Nuclear pore complex (NPC) constitutes the only regular route of cargo transport between the cytoplasm and the nucleus. The vertebrate NPC, with a combined molecular mass of over 100 MDa,11–13 consists of three central ring scaffolds that collectively define the central pore: cytoplasmic ring (CR), inner ring (IR), and nuclear ring (NR)4,9,14,15. CR and NR share a similar overall organization and are characterized by a conserved set of nucleoporins. Here we present single-particle cryo-EM structure of the nuclear ring (NR) subunit from Xenopus laevis NPC at an average resolution of 5.6 Å.

The structurally resolved NR subunit contains 22 molecules of 12 distinct nucleoporins, one molecule each for Nup205/Nup93 and two molecules each for the other 10 nucleoporins. Each Y complex comprises a short arm (Nup85, Nup43, and Seh1), a long arm (Nup160, Nup37, and ELYS), and a stem (Sec13, Nup96, Nup107, and Nup133). Compared to the CR, each Y complex in the NR contains an additional nucleoporin ELYS, which closely associates with Nup160 and Nup37 in the long arm. In our structure, the N-terminal β-propeller of inner ELYS stacks against the N-terminal β-propeller of inner Nup160; the α-helical domain of inner ELYS aligns with the α-helical domain of inner Nup160, orienting the AT-hook domain into the nucleoplasm. Through close interactions with Nup160 and Nup37, ELYS becomes an integral component of the long arm of the Y complex in the NR subunit. Notably, inner ELYS from one NR subunit also bridges interaction with an adjacent NR subunit. Unlike the CR subunit, the NR subunit contains only one molecule of Nup205, which corresponds to outer Nup205 in the CR subunit. Similar to that in the CR subunit, Nup205 in the NR subunit interacts with the short arm and the vertex of outer Y complex; it also associates with both arms of inner Y complex. Unlike that in the CR subunit, the NR subunit only contains one molecule of Nup93, which interacts with both stems of the inner and outer Y complexes. Nup93 connects the stems of inner and outer Y complexes within the same NR subunit, and places its N-terminal extended helix into the axial groove of Nup205 from the neighboring subunit.

> MAAQLALNSEASLWGPYREIWQTVLSALIKRQPEAVHSLDIVLKKYKPDFISLFKNPPKSAQQHERVQKASTEGIPIKGTQRTRILEEQLIKEAFILSDLYNIGEIAAVELLLIGEQQQPTFHGLTRGLVAILLYWDGKSCMAESLLHLIQARKGKTFTLDHSPEVVSMVTRFTDDLMEQGLTNKILTLISQIDVNNEFDKLKKERGLGNKKHRKEVSDLIKECQQSLAHSLYSWSCQTPLNREDTLLLIGYLEKVTVEGDGSLDKVNLTLLMSLLYCLDVGFLEQGTDDREELMKQASMFMDRQYIAAIHNRLQNTQPWKSPGMQATVRLAWALALRGISQFSEVLEFSEADEPMAEIAIGGNVFLFLTEAVVGSESFCTDEFFIRRIHKLVTDFPTLMPMKVKQLRNRAEEDARLIQMSMQMGNEPPASLRRDLEHLLLLIGELYRKDPFHLELALEYWCPTEPLQSTSLMGSFLGVAHQRPPQRQVLLSKFVRQMSDLLPATLYLPYLKMLRGLASGPQCAHYCFSLLKANGGSSAENLQAAGGSPVSWDHFFHSLMLYHEHLRRDLPNTDNIHQRHPPLRGITQRELDGLIACLQLTCTIIDWSESARLALCEHAQWMPVVVILGLLQCSIPPLLKAELLKTLAAFGKSPEIAASLWQSLEYTQILQTVRATGLRQGVGIEVELNEIESRCEEYPLTRAFCQLISTLVESSFPTNLGAGLRAPGFEPYLQFLRDTVFLRYRTRAYRRAAEKWEVAEAVLDVFYKLLKDYEPQPEDFVDQYVELQGEERVAFKPPGFSLMHHLLNESPMLELCLSLMEEGVTQLDTYAPFPGKKHLEKAVAYCFMLLNLTLQKENRFMDLLRESHLSMIVTPLEQLLQGINPRSKKADNVVNIARYLCHGNSNAELAFESAKILCSISCNSKIQEKIVGDFTQDQNVSQKLMVGFVSCLDSEEAEELLDSEKEAEDQVKQTNIRYMTKIHILNLLITSLEMKAPNLAMFLLGYELKKPVSTTNLQDSGVLGCPRTCLHSILDILRKGTDVRAGPVAVWDTPHLAELCYQVIYQLCACADTSGPTMRYLRTSQDFLFSQLQHLPFSVEESEISAMNQMSWLMKTATIELRITSLNRQRSHTQRLLHLLLDDMPTRPYSADGEGGMEDESRSLSGFLHFDTTSKVRRKILRILDSIQFSNEIPEPLQLDFFDRSQIEQVIANCEHKNRRGQTVCNVKLLHRVLVAEVNALQGMAAIGQRPLLMEEINTILQYVVERNKLLQCLHAKRHALESWRQLVEIILTACPQDLIPTEHRQLIIRDLLQDLHVKILDDDAAQELMPIVAGAVFTLTAHLSQSVRTELKQPMTASGLGQSQYVQMLDGSFAAPPGTENISAGFASIGDSSLHMILRNLLEFILKTGGGFQRVRAHLYGSLLYYLQIAQRPDEPDTLESAHKSMWERLTAPEDVFSKLQRDNLSIFESYGTALMEVVCRDACDGHDIGRMLALALLDRIVSVDRQQQWLLYLSNSGYLKVLVDSLAEDDVVLRNLLTPQPPLLKALYIYESKMAFLTRVAKSSQGAIELLRSGVIVRLAQCQVYDMRPETDPHGVFGMRETPVFIPAPVERYRQILLPALQICQLILTSSTAQHLQAAGQVLQFLVAHSDTIQAILRSQEGSLGSLQELALLTGIISKAALPGVLNELDIGLNDGSMMELQGHIGRFQRQCLALLNRFGGSDRLRQLSLQDDSSRLDGVSKKDDMELAMQQICSNVMEYCQALMIQNSPSFQQTVCLFTPSLKESASRDGTRQDSQVSILPSWRLPSLGVVIHLLKQSANNFFTYYDIHRQSVGKLQNVEQLPPDEIKELCQSEMPVGADKISTTQKYGLARRRLVKLINSRAKLLSLCSYIIETCLYILWRHLEYYLLHCTTSDSQDPVFSNMTFGNRRFQDTFNTDPNMDPRNLRQNKVSQQDVDTLLREGANSFGESLQKRLLDIESLYCKVRSRHSFIQALVRRIRGLLRVSRV;>MEELDVDPAETPIPGLGQQNRHIGFSWGPGDLLLYETLYQKQGNSETAARCPFMYLVRSDEDIYSPVLRKLFNESHSIFVGLQKSAEEASGKSRKAQLVQVSRNYRSVLRACMEEMHTLSESTRETAQKYISQISILSAMELSWNLCEILFIESAPAGPLLILLLEWVRLHVCEVDNIVQDVLRSEKPTEHEKFWDGVTGYVLQGRMNEARQLLAKEASTSASARSMCRVLDDLLKKMPMLHTGGTQTLTEFELKWQHWREECERHLQNGTFSSNVHMEAVCRVLLGDEEVLLEKRDLMTTWYHFLVSRLLFKHPTVKPTELHFYAQSSLDMFLAGDSCPEPLDNILLAAFEFDIHQVIKEFSIVSSNWWFVAHLTDLLDHCQLFQAHNLYFGANMREFLLLDYASGLFSHHSLWQLGVDYFDYCPNLGREYLKLHMERIPLSTEKKALKALRICEQRQMTEQVRSICKTMAMQSLCNRRLGSALSWSIRAKDAAFATLISDRFLKEYCERGNFTDLDLIDNLGSAMLLSDRLTFLGKYREFHRMYSQEQFSEAASLLLSLMTARIAPCSFWLTLLLDALPLLEQKQVIFSAEQTYELMRCLEDRMAAKLESTSPDEIQKQDSSIDNTKVEMLRLALARNLARAIVTEGALQE[2x];>MADKFAAKFVSHKISRTRWRPVSASSLQQPDVFATGSWDNEENKVCVWATSDFGATSLDEEYQGDPKQLCDIKHPGDVMDMQFLDKERIVTGSSTGTVTIFRHHENNQTLSVNQRWEQAHYHVGSNMRAPCTAIVCSSPEIVSVGEDGRINCFRAESRDVLRTIDDADSSTMHGVTFLRTTEILTVNSVGQLKLWDLRKQGNDPTQIFSVTGERVPLHCVDRHPNQQHVVATGGQDGMLCIWDVRHGKMPMSLLNAHEAEMWEVHFHPSNPDHLFTCSEDGSLWHWDASADSEKPTFLLGGRSTFNISRSSIAPPNANQSLACAWLSTDPTKGQLEITNLLPSSTLSVNSLDVLGQNLVCGTDAEAIYVTRRLFS[2x];>[2x]MFVARSIAADHKDLIHDVSFDFHGRRMATCSSDQSVKVWDKSENVNWHCTASWKTHSGSVWRVTWAHPEFGQVLASCSFDRTAAVWEEIVGESNDKLRGQSHWVKRTTLVDSRTSVTDVKFAPKHMGLMLATCSADGVVRIYEAPDVMNLSQWSLQHEISCKLSCSCISWNPSSSRAHSPMIAVGSDDSSPNIMGKVQIYEYNENTRKYAKAETLMSVSDPVHDIAFAPNLGRSFHILAVATKDVRIFTMKPLRKELSSSGGVTKFENHTVAQFDNHNSQVWRVSWNITGTVLASSGDDGTVRLWKANYMDNWKCIGVLKGDGNPVGNSFQGIFGSSIGSASHGLQNSVNGTSTSGRKHS;>MAAAERHMTPFQAIDWAGSITLPMVQRVGGFTRAIMAASVNLERSYMELIGAERETSRRNFRDLSLRPDVNLVIGGPKYADCAGGYCYSESSSLLSATRNRFLHWTSYADTLELVEISLDINLVNNAVRLRILNCSILPGGVHICETPNNIVVLILTNQTVHRLILPHPSRMYRSEIISDSHIQSIFTDIGKTNFHDPSNTYVIPAIPGRAPNTTASTAWLSSDGEALFALPSISGGILVIKMPPHDMEGLVTIAELKQSSVMQRLLTGWMPSSIRGDQGPAHLPVSLAVHTLDHDSYLFALCQDHKLRMWSYKDQMCLMVADMLEYVPVSKDIRQTAGTGHKLRLAFSETLGILYLGVYLHTPKQGQFCVFQLMCAESNRYSLDHISSIFTNQETLIDFTFTLTSMDIWALWLDDDNQTVVKHINFEENQAGQWNPVFVNPLPEDDLAISDEQEPQEAYLECLFAPGRFTIAAVQKAIQILRKGSGRVLDLSWEELRKDVTLTVENEIQNAVIDYDVSQEEFRQINIENWCKFYTCCLQYQETLSRPLALLVHPDTNMVCLLRKGFLSFLAPCSLVEHLYLVPAEHLLTVDESVISDDIDAASDIVNLIQCLRMIADYISEDMAYLMESACCHLQSPERVAEQILEDLIANDIDNIMENIQNKLQDTRNPIRAIGFLLQNMDYETNADMEQPQPNTRLNLSTLYGSITASSVVCQAICKISATRFLICRDLLILQHLLLRLGDMALIGAGQLLHSQQELIPRAAQLLLSYYMIRWGSQCLACAVPVDILESNLQHLSVLELSDSQVEKRRYTSGIQTIVELFFEDVARKHFPHVFIQSGASQLQEPLNWSDLIKRITNYLLQLLWPSNPNFQFAECLMRNCQYTQLQEYVRLLLPWCQVNVGSCHFMLAQCYLVAGEGHKALDCFSQAASEVEREDFLEKLIRVEEGESVSPRLQYYNRVLRLLEDVGLPELVIQLATIAIGEASDDWRSQAALRTRIFKHHLDMGHNNQAYDALTQIPDPSRQLDCLRQLVVVLCERSQLQDLVEFPYVNLHNEVVGIIESRARAVDLMTHNYYELLYAFHIYRHNYRKAGSVMFEYGMRLGREVRTLRGLQKQVNSYLACLNCLRLIRPEYAWIVQPVSGAVYERPGASPKRNYDGESSAVPSSSQIEILELRDLEKEYVLAQTRLTLAKHNPSTAAIAGSSAAEEMVALLVQAGLFDTAISLCQTFKLALTSVFEGLACKCIRLQQGGEAAQAEAWEWLAANQLATVITTKESSATDEAWRLMISYLDKYEAKNTLYHHCIINKLLSHGVPLPNWLINRYKAMDAAELLRLYLKYDLLEEAAELVLEYVDALLGKGHQYFGIQAPLSATSQLVWFPYSAIDHLRQALGENESNQHNQAILSKLQRKMDEYFQKLKKATDDYKKLVQKPLRA[2x];>[2x]MKQDSASNATYTVDCEDYVHVVEFNPFDSGEAGSLLAYGGISYVVIASCRFQEEDSTVEGIEFKTLKTFHHGERVVAIAWSPETRCDALLPLLRFATAAGDKKIRIFTSDFQDKNEYKVIEGHSGYINDLVFCSPEGTDIASVGDDHTCRIWDLDGKQIAMFILRSPGMSVAWHPEGAFKLMVAEKTGTIRFYDLTTHQAILSLESVQVPLMSADWCVRNTLRIGAVAGNDWIIWEMPRSSYPQDNKPAHADRARMFRWSKCNENVFATTGYPGKMKSQIAIHHLAHPQPILIGTAPVGSGLSWHRRLPLCVVGGYRKLFFWLTEM;>[2x]SKYGLQDSDEEDDQLNNAEAKKLKAAPVPPQGKPPPLQQATLPGKVTPPPQSPAVDQLDRVLELDSDMADITQDQDLDSVAEEQDITEEQEPLSASSHIASSLGINPHALQVMKASLLLEEEDGEMINRFSSFPSSMDPYPDVRSPRLFPSSHAKRTSSMGLLQSKFASPSISRISETAQGSHSPRILPVTPWSVPAPLAPTFVIPRPAPETHLRTVGTRRQQELVPLEKSVTHGRGSLLIDMGLFMGRSFRVGWGPNWTLVHNGDKLTERLNAEEDQNMDTIDYGFLPKPTSAKSLTESPFKVHMEKLSLEQKSRELQSYLMPLEIELKNSSVDRSAQCPHFKPNAGVAAIHDYAGWVRNLSNEAGELEAVVKQWGLTWTLCESLWGQLKELEASLDEPNEYVRNLERRKAFSHWLAHTAEERIEEEVSLYGPERHVEAVFSFLTGGRISDACRLAQKSGDHRLSLLLSQMVGSQEMRELISLQLVDWNKLQVDHYIQEERLRVFCLLSGTPVWRSSDNRSINVCSQLDWKRTLAVHLWYMLPPTATIAQALRLYERAFQEHEEGEPYACYPLPPYLEDCSISLGDEPSAKFSSLQRDVCVHLLKLYSERQYDLCQLLDPSSVTPDPLDYRLSWHLWMVLQALNYTHLSEHRQGTLHASYAAQLENVGLWEWAIFVLLHIPHPHIREAGVRELLNRQCVVRESPESLAKENFLIHRLCVPAQWVHEAKAIRSRRDGDRHKEALYLLKGHQWNPCHKLVTRHLAADAVINENYRYLQSFLGELSNPEHCKHIQDWETAGKVYLDYIRVIDMLNLIQQDESSGCELEKLHTKVMSLCKWVELIHCYTAKDRLAQSEMAKRVANILRVVLSLQQPPESMSDSSEPRVPLRLLAPHIGRLPMPEDYALEELRGLTQSYLRELICDS;>[2x]MVSVINTVDTSHEDMIHDAQMDYYGIRLATCSSDRSVKIFDVKNGGQILIADLRGHDGPVWQVAWAHPMYGNILASCSYDRKVIIWKEENGTWEKTYEYTGHDSSVNSVCWAPHDFGLVLACGSSDGAISILTFTGDGPWEVKKISNAHTIGCNAVSWAPSVIPGSLVDQPSSQKPNYIKRFVSGGCDNLVKIWREEDGQWKEDQKLEAHSDWVRDVAWAPSIGLPTSTIASCSQDGRVYIWTSDDAATNCWTPKLLHKFNDVVWHVSWSITANILAVSGGDNKVTLWKESVDGQWACISDVNKGQGAVSTVTEGQLNDQ;>MDMLSPVVREAEVSRAARRQSSNRKNPADESWSNATPTRGPSSRTTGQTLFRQHMTPQTWNSSRPPDVSAILGTVGRSPRLLQTPGRLANLSMMSNPDDSVWTTTFSPGRTGMYTTLDSPSFTEDITLSAVMLQEEDPGEAATMSMYPDFLKSFLEHPSSAVFELIEQYEATCNTQITLLKKIVKRVTPGQQKFSKTASILWLLQQEMVTWRLIAALYRDRIQSALEEENMFEIAAPNASEKTIVDKLFQRDTLVRQSQLVVDWLESIAKDEVGDFSDNIEYYAKSVYWENTLHTLKQRSMLSLGSSRPLVSELDPDAPIRQKLPLDDLDREDDIRLLKYLFTLIRAGMTDEAQRLCKRCGQAWRAATLEGWKLYHDANINGGTELQAVEGNPYRCVWKTCCWRMAEDEQFNKYERAIYATLSGNLKQLLPVCESWEDTVWAHFKVMVDSLVEQEIRASIISFNEANELPREYLEANWTLDSVFEELQATDKKRVLEENREHYHIIQKFVILADVDGLMDEFSEWLSNGKNLLLGHLLRFMTHLLLFFRTLGLQAKEEVSVEVLKTYIQRLINEKQIELIAFYVSHLPQELAISQYAVFLENITDPDQRQRCLELAKEAGLDVASITKTVVENTRKKDAGEFAHHDFAPALDSGTSEEDRAKIDVIDWLVFDPAQRAEALKQSNAIMRKFLASKKHEAAKEVFAKIPQDSIAEIYSQWEEQAMDSALPAEDDNAIREHLCIRAYLESHEAFNEWFKHINSPPQKPTLVGQASFTEKVAHEHKEKKYEMDFGIWKGHLDALTSDVKEKIYNVLLFVDGGWMVDVREDTEEDPERSHQMVLLRRLCLPMMCFLLHTVLHNTKQYKDCLRLADIVSSENQKLYTVFSKTEMRNLLQKLRESSLMLLDLQLDPLGYEIQS[3x];>MFPSPRAQGMGSARRPFNSRLTGGRKALGPGVTASSSPSALYSPVGRRVSASGARSTPSRVYLHPAASETVNYNVQLFGSSLPVKVMEALSNASADEPMAACIHEGGWAWLACNDRLIIWKISHSSSAKLMVCKELPLPLSDSEWSADLVDICAQTGDPAAAQSVALMAATPEGSSRYWPNILHEGTYIESYTEFGSSLCAFVTAVKGNSFILSSEKNQLVRLTPDASGKMNQRVLPQGQGMLSGIGRRVSTLFGILSPAVESTLCSVLWDKGDCFYTLTDSSINKWDLDDTSESQVLNWDMSRVLREYISDAIWGSESDYDDIKAGININYLSLNQNCDGLVILSAAWHPGDNPCQIYYTLVTVKDEGYNISDEITVEVTQFNPVFQARGMQLCQLVVPNFSSQACYLYTQEMIFACSTGTGRSTLPQEKIPFEAQGDNIVGAGSCEGWPVFFIRKSGMLTVVARETASVLPEHMEESLSSVSKSSRQAVVKDSRPDQIAHDDKTKHLKAAFLRYCRKDILGAQSMVDSLFSDSDMEPDDELDLAVNQISVDLIDDYPASDPRWAESVPEEAAGFSNTSLILLHQLEDKMKAHSFFVDFLHQVGLFSRLSTCQTKGMLVATRLLLSEHAEKLSAAIVLKNHHAKLPVLVNSAIQLALDKRMCTVPQNLTAADVYFREVSQMEIIFECLVDKEEADLESTSIDSVEWANIVVNVNTILKDMLHVACQYRQSKNSLYKNESGIQEPEHVPWTASSGTAGIRSVVTRQHGIILKVYPQADSGLRTILIEQLAALLNYLLDDYVTQLKSIDKLANEERYNILEMEYAQKRSELLSPLLILGQYAWASNLAEKYCDFDILVQICEMTDNQSRLQRYMTLFAEQNFSDFLFRWYLEKGKRGKLLSQPASQHGQLAAFLQAHDHLSWLHELNSQEFEKAHRTLQTLANMETRYFCKKKTLLGLSKLAALASDFQEDVLQEKVEEIAEQEHFLLHQETLPKKLLEEKQLDLNAMPVLAPFQLIQLYVCEENKRANENDFMKALDLLEYIGDDSEVDVEELKLEILCKAIKRDEWSATDGKDDPIEATKDSIFVKVLQNLLNKGIELKGYLPKAETLLQSEELNSLKTNSYFEFSLKANYECYMKMQS[4x];> MPSATPGAPAASAAMQEALEGAGRIIDRLLQEDRAYPDLSELLNVPVHTCPTISGVSEMDYPLQSPGLLTIPSLPEISAIRRVPLPPELIEQFGHMQCNCMMGVFPEISRAWLTIDSDIFMWNYEDGGDLAYYDGLSETILSVGLVKPKTGIFQPHIRFLLVLSTPVDIVILGLSFANLQPGNLNDSISGGMQLLPDPLYSLPTDNTYLLSITSTDNGRIFLSGKDGCLYEVEYQAEAGWFSQRCRKINHSKSSLSFLVPSVLQFAFSEDDPIVQIAIDNSRNILYTRSEKGVIQVYDLGVDGHGMSRVASVSQNSLVSAAGNIARTIDRNVFKPIIHISVIEMSESVNCHLLAVTHTGVRFYFSTVPFKQPTARPCMLALVHVRLPPGFSASSNVEKPSKVHKALYNNGVLLMAASENEDNDMLWCINRDSFPFQKPMMETQVTTQVDGHSWALSAVDEQKADKIVTPLNKDLIPLTDSPVIIQQHMIPPKRFVLLSAQGSHIFYKLRPVDQLRHLLVSNSGGDGEEIERFFKLHQENQACATCLILACSSAASDREVSSWAARAFFRYGGEAQLRVQSALHAPSNVGPIFGSPLPVASPIPVGSPMPNPSFLGTPTQGACPPNVSTPAYGVATPAPQPPAVPGMMGTEIVFSGKHNGICIYFCRIIGNIWDGSVAVENTFQSGNREVTAIDSSVTPQHLESVLKELKGLLEFLDRYSQFTAGSLGNPGFGTPANRQQRLVSLGRPDIGSSQQAQQELQRKYHTEAQLAEQFSLQGIHQLVRKMCQALALWKLLCEHQFSLVVSDLQKELQEQLKITTFKDLVIRDKELTGALTASLISCYIRDNASVDGISYRLQEVCPLLYSTDDAVCSKANELLQRSRHVPNKQEKERMLRESLKEYQKISQQVDLPNVCAQYRQVRFYEGVVELCLSAAEKKDPQGLGLHFHKNGEPEEDMAGLQAFQERLNSYKCITDTLQELVNQSKAAPQSPSVPKKPGPPVLSSDPNMLSNEEAGIHFEQMLKLAQRSADELFNIALFNWLIQADLTDKLLELNSPFLEPHLVRMAKLDQNKVRYMDLLWRYYEKNRNFSNAARVVAKLADMHSPEISLKQRLEYISRAILSAKSSTTMSTLAADGEFLHELEEKLEVARIQLQIQETLTRQYSHHSTVGDAVSQLDSQLMDITKMFGQYADPFRLSECKLAIIHCAGHSDPILVQTLWQDIIDKELSDSMGNSSVDRMQSLHLKITSLGKIYASTPRYFPLEFLVKYLEQQVCNFSWDAGFVTYTMQEINVPVPKLLEVYDHLFKARDPWWSRMKKPLHLLESIYILLSGYVQEPSKVPSYERRRFTTLCLDAISCYLVELQSMDPAPALLNTVSNFKSLQAKLERLS;>MDGEGFGELLQQAEQLAAETEGVTELPHVERNLQEIQQAGERLRSKTMTRTSQESANVKASVLLGSRGLDISHISQRLESLSAATTFEPLEPVKDTDIQGFLKNEKDNALLSAIEESRKRTFVMAEEYHRESMLVEWEQVKQRVLHTLLASGEDALDFTQESETSYISESGAPGRSSLDNVEMAYARQMYMYNEKVVSGHLQPSLVDLCTEAAERLDDKNVSDLWVMVKQMTDVPLIPASDTLKSRCSGQMQMAFVRQALNYLEQSYKNYTLISVFANLQQAQLGGVPGTYNLVRSFLNIRLPTPIPGLQDGEIEGYPVWALIYYCMRCGDLMAAQQVVNRAQHQLGDFKNCFQEYIHNKDRRLSPTTENKLRLHYRRAVRASTDPYKRAVYCIIGRCDVSDNHSEVADKTEDYLWLKLSQVCFEDEANSSPQDRLTLPQFQKQLFEDYGESHFAVNQQPYLYFQVLFLTAQFEAAIAFLFRLERTRCHAVHVALALFELKLLLKSTGQSAQLLSQEPGEPQGVRRLNFIRLLMLYTRKFEPTDPREALQYFYFLRNEKDNQGESMFLRCVSELVIESREFDMLLGKLEKDGSRKPGAIDKFTRDTKTIINKVASVAENKGLFEEAAKLYDLAKNPDKVLELTNKLLSPVVSQISAPQSNRERLKNMALAIAERYKSQGVSAEKSINSTFYLLLDLITFFDEYHAGHIDLSFDVIERLKLVPLSQDSVEERVAAFRNFSDEIRHNLSEILLATMNILFTQYKRLKGSGPTTLGRPQRVQEDKDSVLRSQARALITFAGMIPYRMSGDTNARLVQMEVLMN[2x];>MQNLEAQVTGSLVAFPDVTQKALKEDEINLDSVLRGKFSTGRTSLAWLACGPQLEITNSVTGERISAYHFSGLTERPPVVVAVKEFTWQKKTGLLVGLVEAEGSVLCLYDIGISKVVKAVVLPGSVTAVEPIINHGGASASTQHLHQSLRWFFGVTAVVTDVGHVLLIDLCLDEVSSNQDELDASDLEVMSVIPTKIPKLREAATRERRHLCLQLAAPTGTTVSCLSYISRTNQLAVGYSDGYFSLWNMKTLRRDYHVQIEGGRVPVCAVAFQEPENDPRNCCYLWAVQSSESGGDVSLHLLQLAFSDRKCLASGQIMYELLEYCEERYSLDLSGSTLSLRGQSNNTKLLGCQTIEKFRVHGEREDGVHEVTSPDTSVSVFSWQVNTYGQGKPSVYLGVFDINRWYQAQMPDSLRSGQFLRNCSYFAFWSLEAVVNITTQDIIFDILVHERSLSRGIPPSYPPPEQFYYPSTYNFDATCLLNSGLIHFACTGFQKETLHFLKKSGSSLNEAIPDGYNRCLAAGLLAPKFTDVQASSLSQEEQLQAILAAAVETSSLGLLTSCIKRWTAEEQPRSAANLRFVLEWTWKKVTLTKQEFDRLCFRLFDGSCNFIDPHTLQSLQQCHLYFSNLTAVLNCFIAQAKEVTQQGAVDLTNKQSVTRLLTLYASVVLWFCRSGMLPDSSDETVQLTRPFYNYQVIQQYYSDQRKKLERLARGKWDTSSLMIDGLINQFGDRIQQLWSRDDNGTGKYPPANLHALLDVYLLENADEMSKHAITIYFLLDIMYSFPDKPDSSIESFPTAFFVPGSLIKLIQGFWLLDHNDYQNSVDCILNPASSRVMSWQHSQIIENLLCHGDSRQALRYLQVMKPVATTSKEVKLHMTVLLANRSILEAWNLQRLHSSRLNVEELLKHMYEMCQEMGLIEELLKLTFTDFEQGYLHKFLQTTGVQNQELLLVHHLQRANYISALQLNQSLKTNHLNDCDRRLRERSGARNAILDQYGKILPRVQRTLASERAKPYSLPSLVWREVARPKPLSTTAKQAAPGSIITKANFICNVLSKIKEVSTANEKREEYSPYQSMVSEEPTAPPLQDIDVPDAFFGTPINKSRRVSRLLDSVVHPVLMEPTPLTSSDTDNNQTPHKSPLLKTSSPLHSSLRRIAHMRSFAKASEFSLLETPLVVRKAKALAANTASSGYTSITPQSILRSSVRTTPLVSPSVSPGRSLTPPLRPKETKISFMELSFTRHAKAAHSSEGNLLAISPVLRSSPDAVWSVKGKVASFTQNTPVKKLDEIDASSSGIQEESQDEMEVSKEISNISVRSEQASLEYHDAPTPEDLENDEISGTTNSQPQVNEVHHQMEDGQLTEKPAELALTEMQEEFIDSEEREIEYISAPLNGPNALECMTAVPDIYLEDASQCILETPEGSSVSVTGEQECVSSAKDSESVISIHDSDDAHSNLSENDQDSEEIEENNLRVPTTVTRCEEFDLIETKDLEVELEEADSEKTNYKDIYPDATVQLGFTVESIEQRYTCELADRRETPSETDEIEGEHFETENNFSLVLEGDVTEEEILEPSSSKTDLELTRPPIAHQKLISENRENIENCETTEKIPANMSPLVDSDHESKTLETLPSEADLSVAEKVLKGTEEKDVPPEVHSEVVLESKLVGNAMMSLDSSESQEVIISQYDNVISIEKLEMTQEKMYGEKTEQINEGQVSPNRDQSTLVKPLTPRRSIRKSSKPADSSTDIIGNITLPTTPKRGLKKAKENVDTLKNSISVVPEEELTLGTRRITRKATLTALDNPEPLQIKEPPSGEDLQVQPSTPTRGRRGKVITSDDLKEPPSGEDLQVQPSTPTRGRRGRVITSDDLREPPPGEDLQVQPSTPTRGRRGRVITSDDIKESPSVEDLQVQPSTPTRGRRGKVITSDDIKEPPSVEDLQVQPSTPTRGRKGKVITSDDIKEPLSGEDLQVQPSTPTRGRKGKVITSDDIKEPLSEEVLQEQPSTPTRGRRGRVITSDGKGYECVEEKNALPLTPTRITRSKNILEPEKGISQIEPEKGISQIEPDKGLSQIEDTGETEHEVVTPRRGRRGKRVVNELVKHFERNSSQPNIKADTSPPVSPKKVSLRWTRTRSENQRINATEEQASKIQEDLSDTPRKRYKKSSNKMGFEETTDTVTEGAIVEDVQESLIISHLGKNPNTSIVRSARKTALPPVTEDHSEQPLLPPESHSKVHSSLAIADEENKTNTRTRSGNKSSVDVSAITFEFSTPKARTKKTAKGSAVPTELIPSTQYVFSPPSTRTRRATRANVSEAVIEPQLQFQESCEIAETEVPEVPASKPRGRPPKHKAKAVTRVLKKPSWSTPPVEIKLISPPESPAVSETNTKTDSTEAKGAEKISVRRTRRRIIAKPVTRRKMR[2x]>[2x]XEFIAWL

Here, we identify an evolutionarily conserved hexapeptide sequence as the major aggregation-prone region (APR) of gastrointestinal peptides of the glucagon family: xFxxWL. We determine nine polymorphic crystal structures of the APR segments of glucagon-like peptides 1 and 2, and exendin and its derivatives. We propose that the pH-dependent changes of the protonation states of glutamate/aspartate residues of APRs initiate switching between the amyloid and the folded, monomeric forms of the hormones. Our results highlight the dual role of short aggregation core motifs in reversible amyloid formation and receptor binding.

Crystals of APRGLP1 grew only at a low pH (pH ≈ 2, T = 37 °C) where the N-terminal glutamic acid self-converted to a pyroglutamic acid (pE) via a spontaneous ring closure. To avoid this side reaction and study the effect of protection of the N-terminal, we synthesized and crystallized its N-terminally acetylated form, Ac-EFIAWL. This compound showed similar spectral properties to APRGLP1. In the structure of APRGLP1 the hydrophobic residues (Phe, Ile, Ala, Leu) form a hydrophobic core, while Trp and pGlu participate in H-bonding with each other and water molecules. A similar interface can be found in the structure of its N-acetylated form. The presence of the acetyl group and Glu instead of pGlu resulted in a lateral shift between adjacent β-sheets, allowing Glu to form H-bonds with waters located near chain termini and Trp side chains from neighboring β-sheets. The fact that this structure also belongs to class 7 suggests that the hydrophobic residues are the main determinants of the topology of the nanostructure. In the crystal structure of Ac-EFIAWL, the interaction between Phe residues from neighboring sheets is made possible by a slight shift of the sheets compared to the structure of pEFIAWL.>MTIDINKLKEELGLGDLAKSLEGLTAAQKAQEAERMRKEQEEKELARMNALVSKAVGEDRQKLEQALELVKSLDEKSKKSAELFAQTVEKQQETIVGLQDEIKSLLTAREGRSFVGDSVAKALYGTQET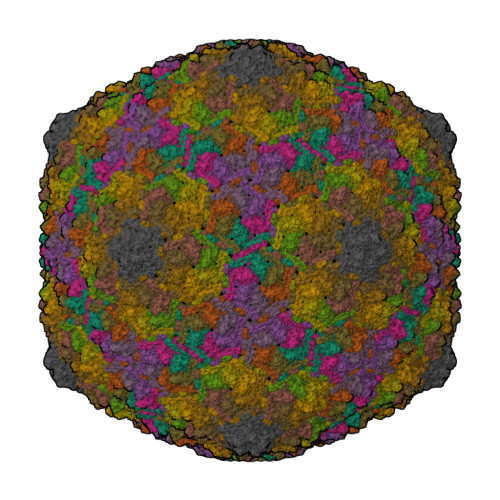FEDEVEKLVLLSYVMEKGVFETEHGQKHLKAVNQSSSVEVSSESYETIFSQRIIRDLQKELVVGALFEELPMSSKILTMLVEPDAGRATWVAASAYGSDNTTGSEVTGALTEIHFSTYKLAAKSFITDETEEDAIFSLLPLLRKRLIEAHAVSIEEAFMTGDGSGKPKGLLTLASEDSAKVTTEAKADGSVLVTAKTISKLRRKLGRHGLKLSKLVLIVSMDAYYDLLEDEEWQDVAQVGNDAVKLQGQVGRIYGLPVVVSEYFPAKAAGKEFAVIVYKDNFVMPRQRAVTVERERQAGKQRDAYYVTQRVNLQRYFENGVVSGAYAAS[13x]>[4x]GPEKEWVEQDEPGVYITLTALAGGARDLKRVRFSRKRFSEIQAEQWWADNRGRVYEQYNVRMV;>GPKWVKTDSDFIVLEI[4x]

Here, we identify RCC1-like domain (RLD) proteins as LZY interactors and reveal that RLD is a regulator of polar auxin transport that controls the abundance and localization of the PIN protein in various developmental processes including GSA control. Structural analysis of the complex of CCL domain of LZY and BRX domain of RLD, which are responsible for the direct interaction of these proteins, reveals hydrophobic and electrostatic interactions at the interface of the anti-parallel intermolecular β-sheet. We also demonstrated that the CCL domain of LZY and the BRX domain of RLD form a complex with high affinity in vitro and that they are necessary and sufficient for the recruitment of RLD from the cytosol to the PM. Our results prompted us to propose a model in which LZY3 recruits RLD1 to the PM of the columella cell in a polarized manner according to the direction of gravity following amyloplast sedimentation.

We found that the BRX domain and the CCL peptide form a 1:1 complex with a KD value of 9.7 nM. To elucidate the structural basis of the interaction, we determined the crystal structures of the RLD2 BRX domain bound to the LZY3 CCL peptide (referred to as the RLD2-LZY3 complex) at 1.35 Å resolution. The RLD2 BRX domain adopts a compact α + β structure comprising an N-terminal three-stranded antiparallel β-sheet and C-terminal α1- and α2-helices. The LZY3 CCL peptide is folded into a β-hairpin structure and docks into the hydrophobic groove between the β3-strand and the α1-helix of the RLD2 BRX domain by forming an antiparallel intermolecular β–β association between the βB-strand of the CCL β-hairpin and the β3-strand of the BRX domain. This results in structural extension from the three-stranded β-sheet of the BRX domain to a five-stranded antiparallel β-sheet in the complex, which creates an additional hydrophobic core comprising nonpolar residues (Trp275, Ile283, Leu285, and Ile287) from the CCL β-hairpin and the surface nonpolar residues (Leu1031, Val1034, Phe1036, and Trp1050) from the BRX domain. The complex is also stabilized by polar interactions and the electrostatic surface potential of the BRX domain is complementary to charged residues of the CCL hairpin. At the interface, salt bridges between charged side chains from the CCL hairpin and the BRX domain are formed (Glu286-Arg1033 and Lys277-Glu1047), and the CCL hairpin loop is stabilized by Arg1038 from the BRX domain. Our mutational analysis suggests a dominant contribution of hydrophobic interactions to the complex formation and the importance of Arg1038-mediated stabilization of the hairpin loop. Here, we have provided the first structural basis for the BRX domain as a protein–protein interaction domain that forms a 1:1 complex with LZY CCLs. The BRX domain is folded into a compact globular structure, although it is composed of only ~60 residues.> MAQPSAGETQASENITLSLLDRIIAEGRMAHDDSQQDYARDMLAEFATQVLDEGMAIDKDTVSMINDRIAQIDALIGAQLDEILHHPELQKLEASWRGLHMLVKNTETGARLKLRLLNVTQKELLIDLEKAVEFDQSALF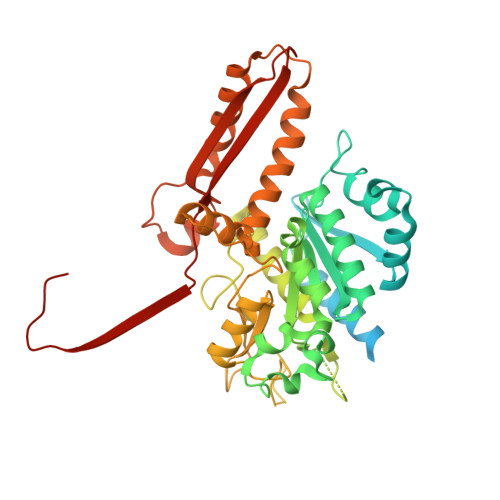KKIYEEEYGTFGGHPFSLLVGDYSFGRHPQDIGLLEKLSNVAAAAHAPFIAAASPRLFDMGSFTELAVPRDLAKIFESQELIKWRAFRESEDSRYVSLVLPHVLLRLPYGPDTCPVEGMDYVEDVNGRDHARYLWGNAAWALTQRITEAFARYGWCAAIRGVEGGGAVEGLPAHSFRTSSGDLSLKCPTEVAITDRREKELDALGFIALCHKKNSDLAVFFGSQTTNRPRVYNTNEANANARISAMLPYVLAASRFAHYLKVIMRDKVGSFMTRDNVQTYLNNWIADYVLINDNAPQEIKAQYPLREARVDVSEVVGKPGVYRATVFLRPHFQLEELTASIRLVATLPPPAAA> M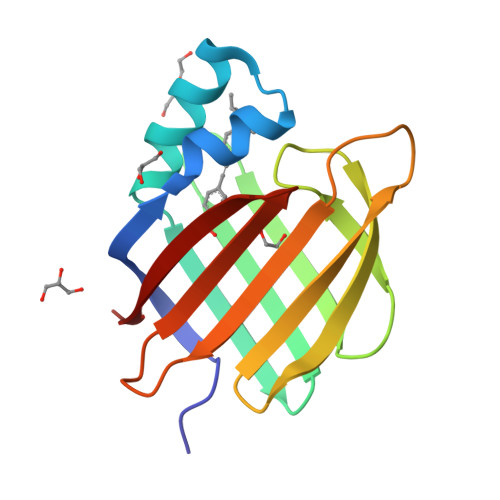PNFSGNWKIIRSENFEELLKVLGVNVMLRKIAVAAASKPAVEIKQEGDTFYIKTSTTVRTTEINFKVGEEFEEQTVDGRPCKSLVKWESENKMVCEQKLLKGEGPKTSWTRELTNDGELILTMTADDVVCTRVYVRE> MRERPHTSGHHGAGEARATAPSTVSPYGPEARAELSSRLTTLRNTLAPATNDPRYLQACGGEKLNRFRDIQCRRQTAVRADLNANYIQVGNTRTIACQYPLQSQLESHFRMLAENRTPVLAVLASSSEIANQRFGMPDYFRQSGTYGSITVESKMTQQVGLGDGIMADMYTLTIREAGQKTISVPVVHVTNWPDQTAVSSEVTKALASLVDQTAETKRNMYES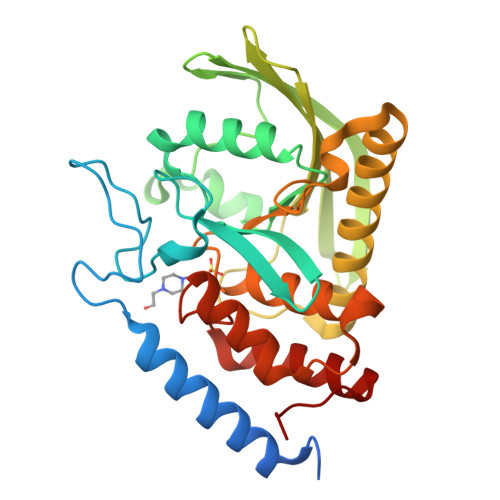KGSSAVADDSKLRPVIHCRAGVGRTAQLIGAMCMNDSRNSQLSVEDMVSQMRVQRNGIMVQKDEQLDVLIKLAEGQGRPLLNS>MAHHHHHHVGTFENITAAPADPILGLADLFRADERPGKVDLGIGVYKDETGKTPVMTSVKKAEQYLLENETTKTYLGLDGLPEFGRCTQELLFGKGSALINDKRARTAQTPGGSGALRVAADFLAKNTSVKRVWVSNPSWPNHKAIFNSAGLEVREYAYYDAENHTLDFDALINSLN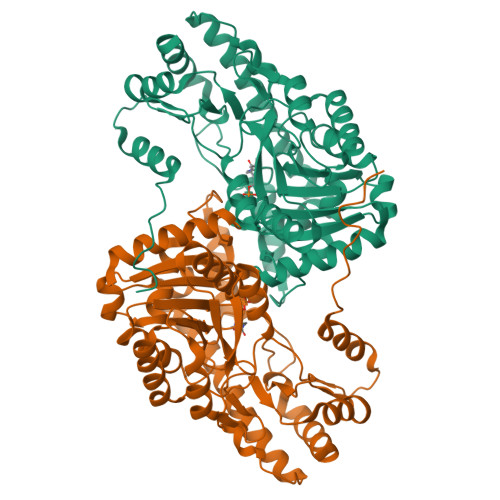EAQAGDVVLFHGCCHNPTGADPTLEQWQTLAQLSVEKGWLPLIDFAYQGFGRGLEEDAEGLRAFAAMHKELIVASSYSKNFGLYNERVGACTLVAADSETVDRAFSQMKAAIRANYSSPPAHGASVVATILSNDALRAIWEQELTDMRQRIQRLRQLFVNTLQEKGANRDFSFIIKQNGMFSFSGLTKEQVLRLREEFGVYAVASGRVNVAGMTPDNMAPLCEAIVAVL[2x]HADACIDIN | C3 H5 N O4 | 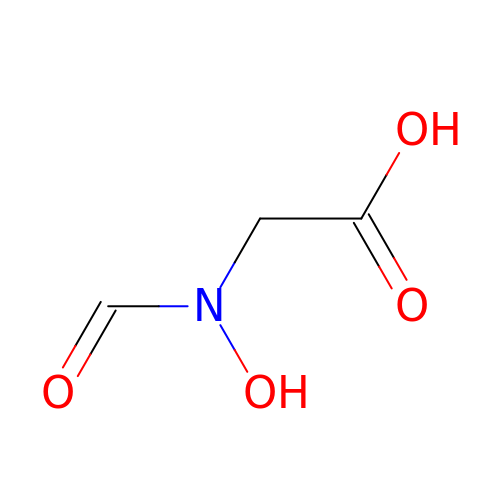URJHVPKUWOUENU-UHFFFAOYSA-N> HMSLSVANSTYETTALNSQKSSTDQPNSGSKSGQTLDLVNLGVAANFAILSKTGITDVYKSAITGDVGASPITGAAILLKSDEVTGTIFSVDAAGPACKITDASRLTTAVG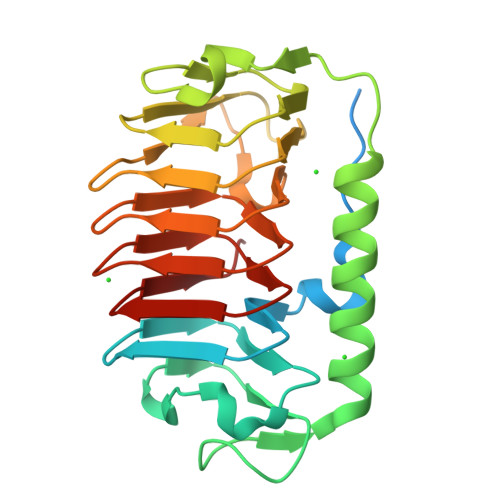DMQIAYDNAAGRLNPDFLNLGAGTIGGKTLTPGLYKWTSTLNIPTDITISGSSTDVWIFQVAGNLNMSSAVRITLAGGAQAKNIFWQTAGAVTLGSTSHFEGNILSQTGINMKTAASINGRMMAQTAVTLQMNTVTIPQ> METCENVDCGPGKKCRMNKKNKPRCVCAPDCSNITWKGPVCGLDGKTYRNECALLKARC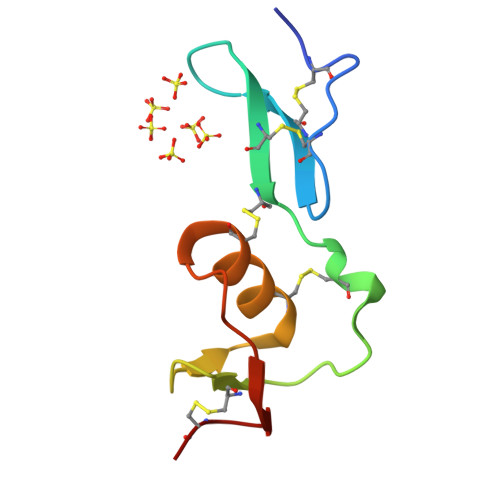KEQPELEVQYQGKCK> MEAVLFDFNGTLIFDTPLHAFCWKEM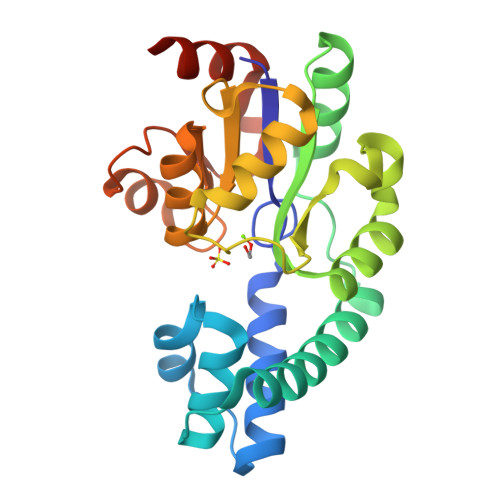AKRIRGTPLSEDEFKLLNGRTNKQLIEHILNKEISDEDAKKYAEEKENLYRTMLMKSDIKLCDGAINLFEALKKCNIPFTIATSSDWGNVQVFIQKYHLEEWFDIDKIIFNDFTFKGKPAPDIYLKASKKLGVSISHCIVFEDTISGIHSALSAGATPIGIASEMTVNELLQIKGCNLAIHTFNEITIEEMVDLIKNKGHHHHHH> MGSDKIHHHHHHENLYFQGHMSQWQAKQELAEAKKTATTFLNVLSKQEFDKLPSVVQEASLKKNGYDTKSVVEKYQAIYSGIQAEGVKASDVQVKKAKDNQYTFTYKLSMSTPLGEMKDLSYQSSIAKKGDTYQIAWKPSLIFPDMSGNDKISIQVDNAKRGEIVDRNGSGLAINKVFDEVGVVPGKLGSGAEKTANIKAFSDKFGVSVDEINQKLSQGWVQADSFVPITVASEPVTELPTGAATKDTESRYYPLGEAAAQLIGYTGTITAEDIEKNPELSSTGVIGKTGLERAFDKELRGQDGGSLVILDDKENVKKALQTKEKKDGQTIKLTIDSGVQ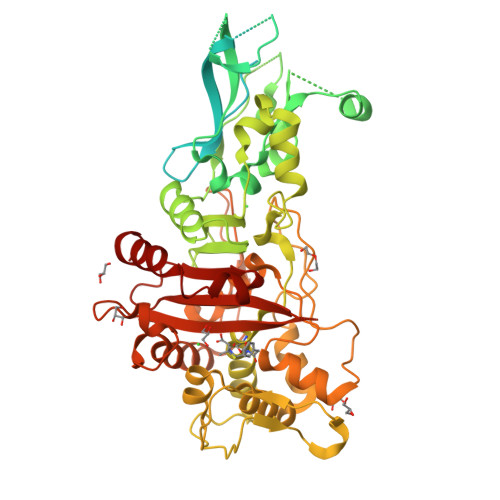QQAFAIFDKRPGSAVITDPQKGDLLATVSSPSYDPNKMANGISQKEYDAYNNNKDLPFTARFATGYAPGSTFKTITGAIGLDAGTLKPDEELEINGLKWQKDKSWGGYFATRVKEASPVNLRTALVNSDNIYFAQQTLRMGEDKFRAGLNKFIFGEELDLPIAMTPAQISNEDKFNSEILLADTGYGQGQLLISPIQQATMYSVFQNNGTLVYPKLVLDKETKKKDNVISANAANTIATDLLGSVEDPSGYVYNMYNPNFSLAAKTGTAEIKDKQDTDGKENSFLLTLDRSNNKFLTMIMVENSGENGSATDISKPLIDYLEATIK We previously showed that LJ0536, a cinnamoyl esterase purified from L. johnsonii N6.2, is active towards a variety of substrates including short acyl chain aliphatic esters and phenolic esters. The structure showed a canonical α/β fold characteristic of esterases, and the enzyme is dimeric. Two classical serine esterase motifs (GlyXSerXGly) can be recognized from the amino acid sequence, and the structure revealed that the catalytic triad of the enzyme is formed by Ser106, His225, and Asp197, while the other motif is non-functional. The structure revealed a prominent inserted α/β subdomain of 54 amino acids, from which multiple contacts to the aromatic acyl groups of the substrates are made.

We determined the structure of the active site mutant (Ser106Ala mutant) and also co-crystallized this mutant with ferulic acid, ethyl ferulate, or chlorogenic acid. We validated that the active catalytic triad is Ser106, His225, Asp197, since the Ser106Ala and Asp197Ala mutants displayed no catalytic activity. The apo-LJ0536 structure was crystallized in the presence of protease, which facilitated successful crystal growth (the mutant Ser106Ala was also crystallized in the presence of protease). Overall, we observed no appreciable differences in the backbone structure between the apo wild-type (WT) enzyme and the Ser106Ala mutant (RMSD of 0.33 Å over all 244 Cα atoms). Trp160 of Est1E corresponds to Phe160 of LJ0536, and Phe160 adopts the same conformation in the apo and each of the ligand-bound complexes. The bridge-like structure formed by this residue in LJ0536, which lies on the first hairpin of the inserted α/β subdomain, is present in the same location in both apo and holo structures.

> MGSSHHHHHHSSGRENLYFQGMATITLERDGLQLVGTREEPFGEIYDMAIIFHGFTANRNTSLLREIANSLRDENIASVRFDFNGHGDSDGKFENMTVLNEIEDANAILNYVKTDPHVRNIYLVGHAQGGVVASMLAGLYPDLIKKVVLLAPAATLKGDALEGNTQGVTYNPDHIPDRLPFKDLTLGGFYLRIAQQLPIYEVSAQFTKPVCLIHGTDDTVVSPNASKKYDQIYQNSTLHLIEGADHCFSDSYQKNAVNLTTDFLQNNNAF pmcMarE is a bacterial enzyme that catalyzes a unique 2-oxindole production reaction through monooxygenation of (2S,3S)-β-methyl-l-tryptophan (β-Me-l-Trp). The amino acid sequence of MarE shares significant similarity with tryptophan 2,3-dioxygenase (TDO), a histidine-ligated heme-dependent enzyme that catalyzes the activation and insertion of molecular oxygen by a histidine-ligated heme into the indole ring of l-tryptophan (l-Trp), producing N-formylkynurenine (NFK). TDO and its closely related homolog, indoleamine 2,3-dioxygenase (IDO), catalyze stepwise O-atom transfers, completing dioxygenation through two sequential monooxygenation reactions. However, MarE diverges functionally by catalyzing only a single monooxygenation reaction on a tryptophan metabolite, terminating the oxidation process before full dioxygenation. To elucidate its enzyme-substrate interaction mode, we present the first X-ray crystal structures of MarE in complex with its prime substrate, (2S,3S)-β-methyl-l-tryptophan and cyanide at 1.89 Å resolution as well as a truncated yet catalytically active version in complex with the substrate at 2.45 Å resolution. These structures establish MarE as a member of the heme-dependent aromatic oxygenase (HDAO) superfamily and reveal its evolutionary link to indoleamine 2,3-dioxygenase (IDO) and tryptophan 2,3-dioxygenase (TDO).

MarE Δ(270–284) was crystallized in the presence of 10 mM β-Me-l-Trp but without the inclusion of sodium cyanide. Unlike the successful crystallization of the full-length protein in the ternary complex, we resolved an ES crystal structure of truncated MarE Δ(270–284) at 2.45 Å resolution through co-crystallization with β-Me-l-Trp. Unlike the ternary crystal, the MarE Δ(270–284) crystal belongs to a body-centered tetragonal space group (I422) and contains two protomers in the asymmetric unit. The dimer-of-dimer structure was constructed through crystallographic symmetry operations, consistent with MarE's homotetrameric oligomeric state in solution. Each monomer structure is nearly identical to the ternary cyano complex, with an RMSD of 0.54 Å for 243 Cα atoms, though it features a longer disordered region spanning residues 217 to 234. In chain A, two substrate-binding modes were observed at the heme distal pocket. The other (conformation B) is a new orientation where the substrate's amino nitrogen points away from the heme center, while the methyl group points toward it (substrate with cyan carbons). Interestingly, chain B exclusively displays conformation B in the ES complex structure of truncated MarE Δ(270–284). In the binary complex structure, the SLGGR loop is disordered, consistent with the disordered region spanning residues 217 to 234. As a result of the disordered SLGGR loop in the binary complex, Asp124 of the DATG loop remains in a retracted position, no longer interacting with Arg235 of SLGGR.

>[2x]GHMKRSLNPDEPNALLSYDFDRGSNYENVLHLTDALGALVPESETEHPDQRFFQVTHLITEYAWVQVHYELRRAIGHLDEDRYHQAVRMFDRATGLSEVTVQAVRLLTDHLPQHSLLMMRNALPEDATGLDSPGYRNLRRVARPVWKAYEQAVERAGLSLQDVIAQQDDGYDGPRSGGSQSLALVREAMLRLDGSVLGWKQHHLIMVWSQLGGQPGLRKGNEEGDDGLELPQSLGGRSLATLEARSQLALFPELWRAAEDAYWLLGTRHDT>[2x]MRSNLLAFSIVASLGLAQVAHAAEGMWVPQQLPEIAGPLQKAGLKLSPEQLANLTGDPMGAVVALGGCTASFVSPQGLVVTNHHCAYGAIQLNSTAQKNLIKDGFNAPTLKDELSAGPNARVFVLDQITDVTAQAKAAIAGAGNDPLARSRALDAFDKAQVAACEADAGFRCRLYSFSGGNTYRLFRNMEIKDVRLVYAPPGSVGKFGGDVDNWMWPRHTGDFSFYRAYVGKDGKPAAFAADNVPYQPKHFLKFADQPLGADDFVMVAGYPGRTNRYALAGEFNETASFTYPTIAKHYNAVLKMIADAGKADADVKVKYAATAASMNNVAKNYLGQLEGFKRIDAAGQKQAEEAAVLAWLKKQGAAGKPALAAHAQLLKHLDTSKSTRERDLFVGQFNNTSAVGAAITLYRLSIERSKP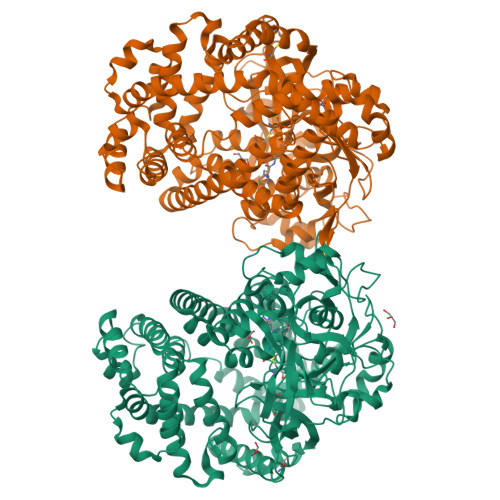DAEREAGYQERDLTTIEGGLKQMDRRYVAKMDQQLQTYWLDQYVALPAAQRDNEVLNKWLAGSDAAAVKSLVNKLGGTELGSLDTRLKWFKADRAAFEASNDPAIQYAVAVMPALLKQEEQKKIREGESLTARPLYLQAVADYKKSQGEFVYPDANLSLRITFGNVMGYGKDGVKYTPFTTLEGVAAKETGEDPFDSPKALLDAVKAKRYGGLEDKRLGSVPVNFLSNLDITGGNSGSPVLDANGKLVGLAFDGNWESVSSNWVFDPVMTRMIAVDSRYMQWIMQEVAPAPQLLKELNLAK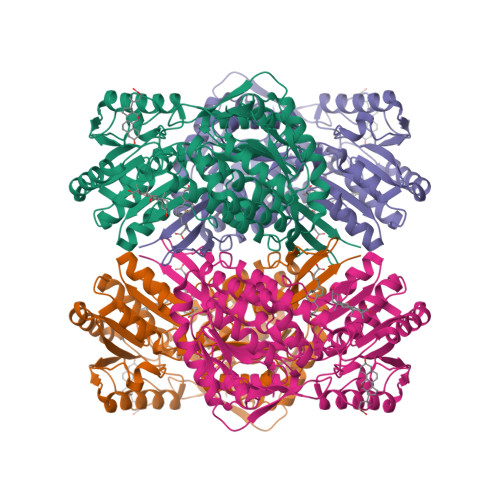> MSVPVQHPMYIDGQFVTWRGDAWIDVVNPATEAVISRIPDGQAEDARKAIDAAERAQPEWEALPAIERASWLRKISAGIRERATEISALIVEEGGKIQQLAEVEVAFTADYIDYMAEWARRYEGEIIQSDRPGENILLFKRALGVTTGILPWNFPFFLIARKMAPALLTGNTIVIKPSEFTPNNAIAFAKIVDEIGLPRGVFNLVLGRGETVGQELAGNPKVAMVSMTGSVSAGEKIMATAAKNITKVCLELGGKAPAIVMDDADLELAVKAIVDSRVINSGQVCNCAERVYVQKGIYDQFVNRLGEAMQAVQFGNPAERNDIAMGPLINAAALERVEQKVARAVEEGARVALGGKAVEGKGYYYPPTLLLDVRQEMSIMHEETFGPVLPVVAFDTLEEAISMANDSDYGLTSSIYTQNLNVAMKAIKGLKFGETYINRENFEAMQGFHAGWRKSGIGGADGKHGLHEYLQTQVVYLQS>MAEENIIFVGK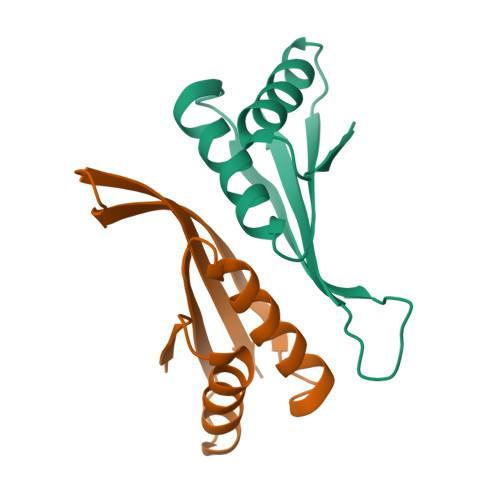KPTMNYVLAVVTQFNNNANKIIIKARGKTISKAVDVAEITRHKFIPDAKYEEIRLDTETLQGERGSSNVSSIEITLSRLEHHHHHH[4x]> MSGFGGGSSGAGSLTQLLATGSMDAALTQNATRTFWKSSYQKHSLFALESINQPFTTQVQFGAESHITVNRQGDLLSWMYLKIVLPGLKVQNQA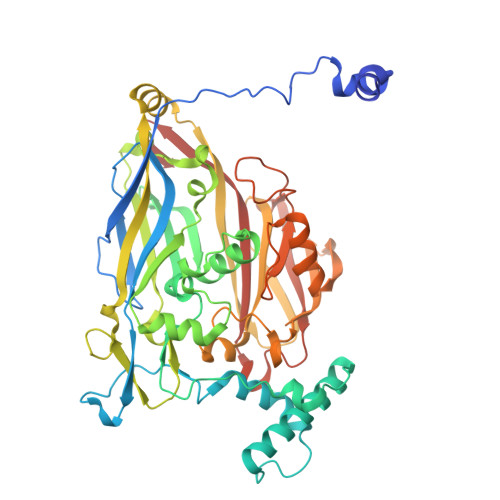DTVQPTQQSFASLDNDVAAQADVSHVLPYIEGAYTEASLNTKEQLIAEAKNSYEAAKYNAAPLPVAAQMQSTEMPDFDYAYWTEAIGFHLIKRAEFKVGGATIDTIWSELLFAMEELMGRAGRRLTETIGRTLRRPTELMKASRQEQILYVPLPWYFTKHPSLAFPLVAATYHNIQLWVQWAQLNSCIIKSRSNLVVLHAERNVPISDDHLRASLECTYVHLEAAERDALTANAGTQLIVQHQAHLQQVSSNNVTARLNFNFPVLEFYYFLRRKANKDAGDHFNFSGIGGRDPVVSAELLFNNTARVTQKPAVWWRAVQALQFHSSAPLTNIYSYSFSLSPEDPITPSGSANFSRLDSVELALTLQDDFGAAHDANSELFVFARSYNILKFTNGLAGLLYSN> DCSSGWSSYEGHC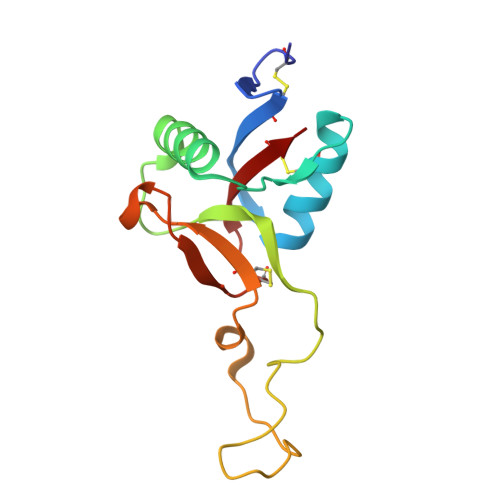YKVFKQSKTWTDAESFCTKQVNGGHLVSIESSGEADFVGQLIAQKIKSAKIHVWIGLRAQNKEKQCSIEWSDGSSISYENWIEEESKKCLGVHIETGFHKWENFYCEQQDPFVCEA>GSHMGGVEVMETVPLSEDTIYKVEAILLPNFASGSNTAVYQSRGAPYTFTDTLDAGSSLCYTLAVVNLPEIPEALCDDTLLVWEAFRVETELIFTPQLGSAGYIRAQGTPAGVEGSQMYFWACGGSPLDVIGINPDPERMNVAAGLEGPSKENQPSVAGIKAT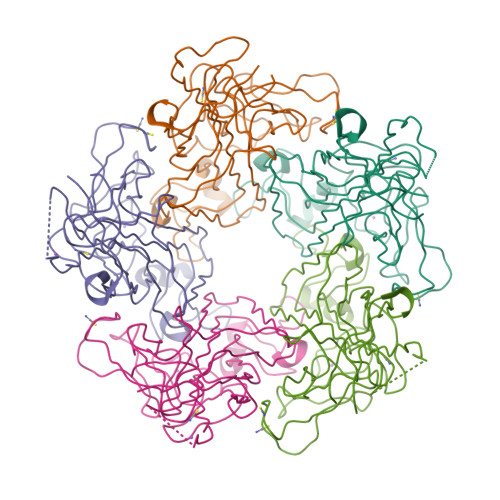RKQVTAANFPIEIWSADPTRNENCRYFGRIVGGSVTPPVVSFGNQSTTPLVDENGVGILCLFGAIYLTSADMLGMVGYAGNPTLSDAYSQQRSVQAAFGRFFRVHFRQRRVKH[5x]> MSLGIRYLALLPLFVITACQQPVNYNPPATQVAQVQPAIVNNSWIEISRSALDFNVKKVQSLLGKQSSLCAVLKGDAYGHDLSLVAPIMIENNVKCIGVTNNQELKEVRDLGFKGRLMRVRNATEQEMAQATNYNVEELIGDLDMAKRLDAIAKQQNKVIPIHLALNSGGMSRNGLEVDNKSGLEKAKQISQLANLKVVGIMSHYPEEDANKVREDLARFKQQSQQVLEVMGLERNNVTLHMANTFATITVPESWLDMVRVGGIFYGDTIASTDYKRVMTFKSNIASINYYPKGNTVGYDRTYTLKRDSVLANIPVGYADGYRRVFSNAGHALIAGQRVPVLGKTSMNTVIVDITSLNNIKPGDEVVFFGKQGNSEITAEEIEDISGALFTEMSILWGATNQRVLVD

In addition to Alrs, a PLP-dependent racemase is found to possess a broad amino-acid specificity (broad specificity amino acid racemase, Bar, E.C. 5.1.1.10). Notably, Lyr is also active against arginine, whereas Bar racemizes arginine, lysine, methionine, serine, cysteine, leucine, and histidine, a useful feature for biotechnological applications. To further develop lyr- or bar-based marker genes with desired properties, we determined the three-dimensional structures of P. putida DSM84 Bar and P. mirabilis Lyr, which are the first structures for lysine-preferred racemases. All structures contain PLP, which confirms their PLP-dependent nature, and the positions of their catalytic lysines and tyrosines are similar to those in Alr structures.

Expression and biochemical characterization of recombinant Lyr has shown that its preferred substrate is lysine. We next solved the Lyr structure by molecular replacement with the Bar structure as the template. One Lyr molecule is found in the asymmetric unit. With the exception of those for the first 36 residues, the positions of all main-chain and side-chain atoms are well defined. Two Lyr molecules associate to form a dimer related by a two-fold crystallographic axis. The tertiary structures of the Lyr and Bar protomers are similar (RMSD = 0.89 Å for Cα positions). The apo Lyr structure has also been established within the internal aldimine linkage. Given the relatively larger space between Thr391 and PLP in Lyr, and Ala393 and PLP in Bar as compared with those in the Alrs, a substrate larger than an alanine may better fit the space. Mutation of the inner-layer Thr391 of Lyr to tyrosine, which is positioned similarly to the conserved tyrosines in Alrs (Tyr354 in BsAlr), reduced the activity of Lyr towards L-Lys to 53%.>MAADHTDVLIVGAGPTGLFAGFYVGMRGLSFRFVDPLPEPGGQLTALYPEKYIYDVAGFPKVYAKDLVKGLVEQVAPFNPVYSLGERAETLEREGDLFKVTTSQGNAYTAKAVIIAAGVGAFEPRRIGAPGEREFEGRGVYYAVKSKAEFQGKRVLIVGGGDSAVDWALNLLDTARRITLIHRRPQFRAHEASVKELMKAHEEGRLEVLTPYELRRVEGDERVRWAVVFHNQTQEELALEVDAVLILAGYITKLGPLANWGLALEKNKIKVDTTMATSIPGVYACGDIVTYPGKLPLIVLGFGEAAIAANHAAAYANPALKVNPGHSSEKAAPGT[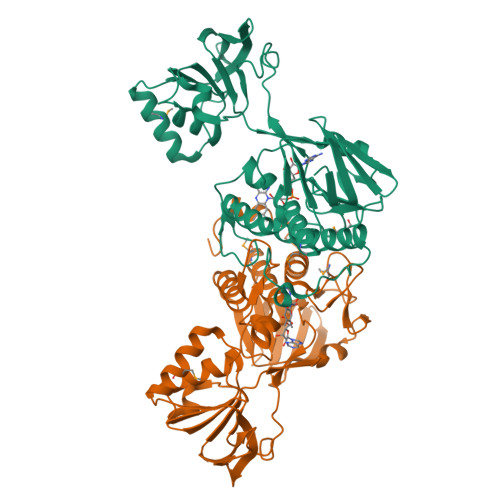2x]>[2x]MERKHHF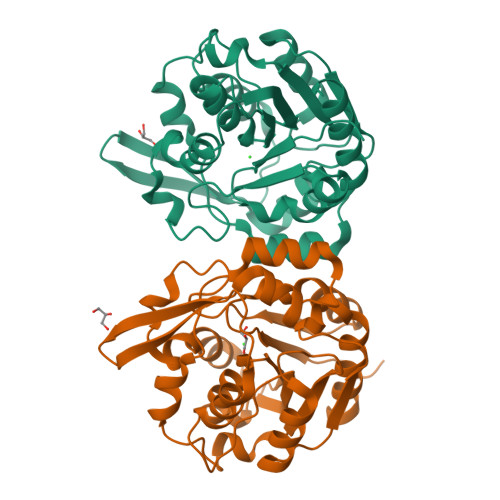VLVHNACHGAWIWYKLKPLLESAGHRVTAVELAASGIDPRPIQAVETVDEYSKPLIETLKSLPENEEVILVGFSFGGINIALAADIFPAKIKVLVFLNAFLPDTTHVPSHVLDKLMEMFGGWGDTEFSSHETRNGTMSLLKMGPKFMKARLYQNCPIEDYELAKMLHRQGSLFTEDLSKKEKFSEEGYGSVQRVYVMSSEDKIIPCDFIRWMIDNFNVSKVYEIDGGDHMVMLSKPQKLFDSLSAIATDYMGL> MGSDKIHHHHHHMKLSDFIKTEDFKKEKHVPVIEAPEKVKKDEKVQIVVTVGKEIPHPNTTEHHIRWIKVFFQPDGDPYVYEVGRYEFNAHGESV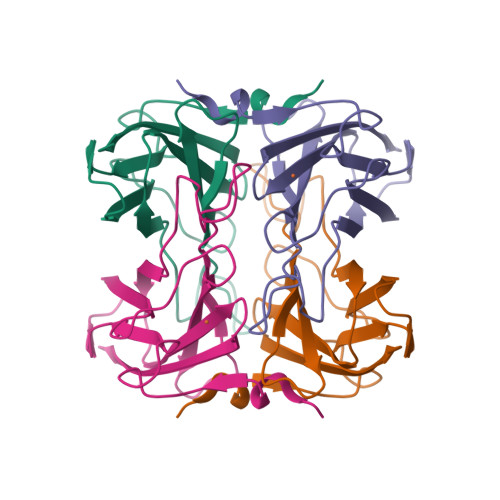QGPNIGAVYTEPTVTTVVKLNRSGTIIALSYCNIHGLWESSQKITVEE>[2x]SNAQFGGLPVPLDQTLPLNVNPALPLSPTGLAGSLTNALSNGLLSGGLLGILENLP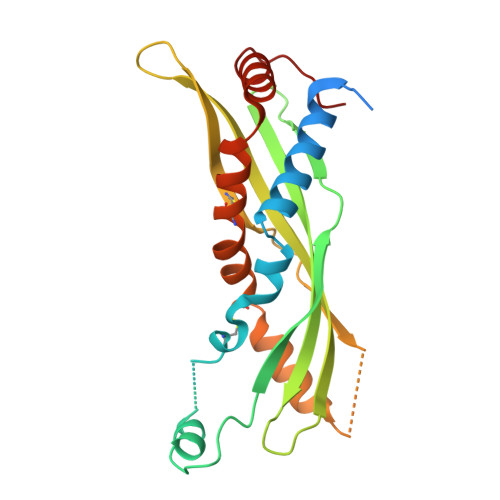LLDCLKPGGGTSGGLLGGLLGKVTSVIPGLNNIIDIKVTDPQLLELGLVQSPDGHRLYVTIPLGIKLQVNTPLVGASLLRLAVKLDITAEILAVRDKQERIHLVLGDCTHSPGSLQISLLDGLGPLPIQGLLDSLTGILNKCLPELVQGNVCPLVNEVLRGLDITLVHDIVNMLIHGLQFVIKV>[2x]MGKGDSIIVAVRVRPFNDREKTRNCKLVIEMPDEETTVIRDPKTNDEKRFTYDHSYWSHDGF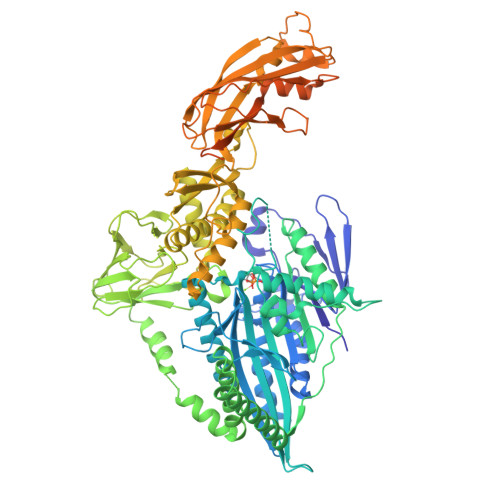SEKKNGYLEPTDPHYADQRRVFEDLGRGVLANAWAGYNCSLFAYGQTGSGKSYSIVGFKNNKGIVPIVCEELFKQIADNKKKNMQFEVFVSMMEIYCEKVRDLLSSTPPPKGGLKVREHPKNGFYVENLTTVPVNSFKEIEAKIEEGTKSRTIAATQMNATSSRAHTIVKITFNQKSSKQAGGTSMKKSEINLVDLAGSERQSAAGTEGDRLKEGIVINQSLTTLGRVIKALHDSQKAKSGKKTQIPYRDSVLTCLLKNALGGNSKTIMIAAISPADINFEETLSTLRFADRAKSIKTNAVVNENQTERALRELREENLRLQSQIQGGTAGDASNEEIEKLRRQLAENQKEMEEMEKSWQQKIAEEAAKHASGASEKVEMEAKKKKMCHLWNLNEDPALTNVIVHFIPVGESVVGNKPTSSGNFIQMSGLSILPQHVTLKNDGNNQIHLSPCSEDLDIFINGKPVHGETQLQQNDRVFFGGNHLYVFNNPTKKGIRTDITYENAQAEIAQNHAAALGNRGLGGGSKRDLILEEELMSTLPLVQRANAMATELGRNVKFEIVLVSPEMRGLTSGLTEIWVKVHNISEDTYFLWEKSRFMNRYYGMQEMYEAKQDGSEDWNMPKERDPFYEPPDSPVFIASSVVFLQSLAYLIDVEEQFPIVDLSGQEIGLLTVGLSPCSTTGKELRGEYVEDPDQLIGKNIAFKVKVISAVGLPRRILKSNCKYRFFGSKKMTTTATVSGNTPAYGHEETFQFKPVTKEVADYLANSNLYITFWGTQRPRGASSRKNSISTIGSNEAREGPNKAKRVERLVHQAKTSENRNISVKALETVLKGVDDNENRKTRKQSMKKAGSTTIKSRSGSKKPKAKGTKLLEVLFQGPHHHHHHGSGSGSWSHPQFEK> MLKQVEIFTDGSCLGNPGPGGYGAILRYRGREKTFSAGYTRTTNNRMELMAAIVALEALKEHCEVILSTDSQ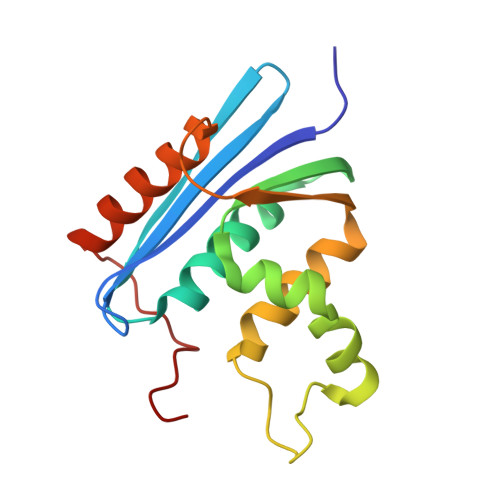YVRQGITQGWIHNWKKRGWKTADKKPVKNVDLWQRLDAALGQHQIKWEWVKGHAGHPENERCDELARAAAMNPTLEDTGYQVEV>[2x]ADPEPCELDEESCSCNFSDPKPDWSSAFNCLGAADVELYGGGRSLEYLLKRVDTEADLGQFTDIIKSLSLKRLTVRAARIPSRILFGALRVLGISGLQELTLENLEVTGTAPPPLLEATGPDLNIL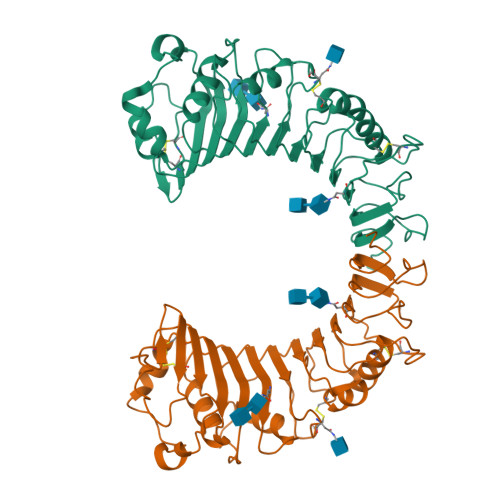NLRNVSWATRDAWLAELQQWLKPGLKVLSIAQAHSLNFSCEQVRVFPALSTLDLSDNPELGERGLISALCPLKFPTLQVLALRNAGMETPSGVCSALAAARVQLQGLDLSHNSLRDAAGAPSCDWPSQLNSLNLSFTGLKQVPKGLPAKLSVLDLSYNRLDRNPSPDELPQVGNLSLKGNPFLDSE>HHHHHHLESTSLYKKAGMATANGAVENGQPDRKPPALPRPIRNLEVKFTKIFINNEWHESKSGKKFATCNPSTREQICEVEEGDKPDVDKAVEAAQVAFQRGSPWRRLDALSRGRLLHQLADLVERDRATLAALETMDTGKPFLHAFFIDLEGCIRTLRYFAGWADKIQGKTIPTDDNVVCFTRHEPIGVCGAITPWNFPLLMLVWKLAPALCCGNTMVLKPAEQTPLTALYLGSLIKEAGFPPGVVNIVPGFGPTVGAAISSHPQINKIAFTGSTEVGKLVKEAASRSNLKRVTLELGGKNPCIVCADADLDLAVECAHQGVFFNQGQCCTAASRVFVEEQVYSEFVRRSVEYAKKRPVGDPFDV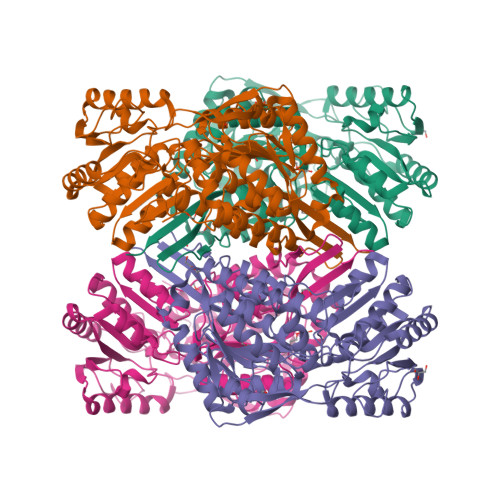KTEQGPQIDQKQFDKILELIESGKKEGAKLECGGSAMEDKGLFIKPTVFSEVTDNMRIAKEEIFGPVQPILKFKSIEEVIKRANSTDYGLTAAVFTKNLDKALKLASALESGTVWINCYNALYAQAPFGGFKMSGNGRELGEYALAEYTEVKTVTIKLGDKNP[2x]> MRGSHHHHHHGSAQDLTNMPSLAPVLKNAMPAIVNVAVQGYLPNNMASGNADDDDGENSKQPSRIPE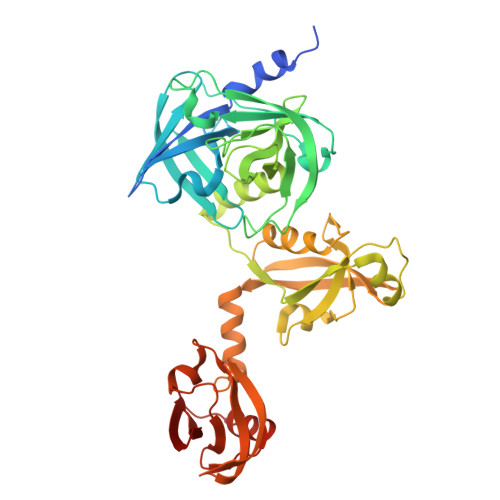KGRKFESIGSGVIIDPKNGIIITNDHVIRNANLITVTLQDGRRLKARLIGGDSETDLAVLKIDAKNLKSLVIGDSDKLEVGDYVVAIGNPFGLNSFGNSQSATFGIVSALKRSDLNIEGVENFIQTDAAINPGNAGGALVNAKGELIGINTAIISPYGGNVGIGFAIPINMAKDVAQQIIKFGSIHRGLMGIFVQHLTPELAQSMGYAEDFQGALVSQVNQNSPAQLAGLKSGDVIVQINDTKITQATQVKTTISLLRAGSTAKIKILRDNKPLTLDVEVTDIKKHEQKLQSNNPFLYGLALRNFEQESPPHGNVVGVQVVGASETSAGWRAGLRPGDIIISANKTPVKDIKSLQAVAHEKGKQLLVQVLRGAGALYLLII>GPGSKPFTLPILTIGELSNSRFPVPIDELYTSPNEGVIVQPQNGRSTLDGELLGTTQLVPSNICALRGRINAQVPDDHHQWNLQVTNTNGTPFDPTEDVPAPLGTPDFLANIYGVTSQRNPNNTCRAHDGVLATWSPKFTPKLGSVILGTWEESDLDLNQPTRFTPVGLFNTDHFDQWALPSYSGRLTLNMNLAPSVSPLFPGEQLLFFRSHIPLKGGTSDGAIDCLLPQEWIQHFYQESAPSPTDVALIRYTNPDTGRVLFEAKLHR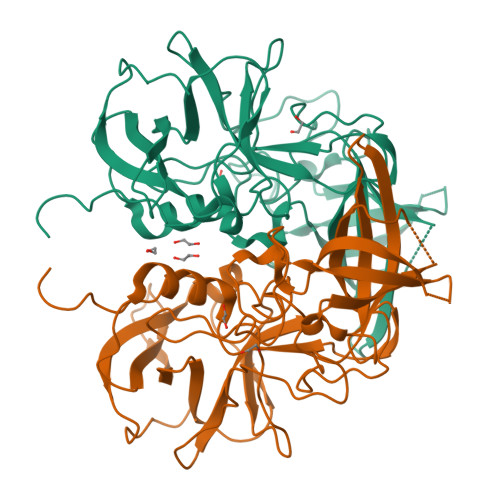QGFITVANSGSRPIVVPPNGYFRFDSWVNQFYSLAPM[2x]Typhoid toxin belongs to the bacterial AB toxin family and consists of two enzymatic ‘A’ subunits, CdtB (cytolethal distending toxin A subunit; nuclease) and PltA (pertussis-like toxin A subunit; mono ADP-ribosyltransferase) linked to a homopentamer of receptor-binding ‘B’ subunit PltB (pertussis-like toxin B subunit), resulting in its unique A2B5 configuration. PltB recognizes the specific trisaccharide motif as its receptor, N-acetylneuraminic acid (Neu5Ac) α2–3 or α2–6 linked to the underlying disaccharide, galactose (Gal) β1-3/β1–4 linked N-acetylglucosamine (GlcNAc) or glucose. The pentameric configuration of the receptor-binding PltB subunit per toxin and the three glycan binding pockets per PltB monomer play an essential role for multivalent interactions between the toxin PltB and glycan receptor moieties. We previously revealed the three glycan-binding sites (BS) per PltB monomer and demonstrated the flexible use of these three binding sites in accommodating glycan receptor moieties that are structurally different.

We also solve co-crystal structures of PltB homopentamer bound to Neu5,9Ac2α2-6Galβ1-4GlcNAc and compare the glycan-binding interface with that for unmodified glycan counterparts. Both unmodified and 9-O-acetylated α2–6 glycans bind only to the BS1. 9-O-acetylated α2–6 glycans bound only to the BS1, while 9-O-Ac α2–3 glycans bound to the BS1 and BS2. Notable differences between the two are H-bonds between the 9-O-acetyl group and Thr65 (via the main chain), as well as between GlcNAc and Lys59 in the interface for 9-O-acetylated α2–6 glycans. These results are in support of the increased binding affinity of PltB to 9-O-acetylated α2–6 sialosides, compared to unmodified α2–6 counterpart. PltB binds to 9-O-acetylated α2–3 glycans (Neu5,9Ac2α2-3Galβ1-4GlcNAc) with a ~14-fold increased affinity compared to its unmodified α2–3 counterpart (Neu5Acα2-3Galβ1-4GlcNAc), while PltB binds to 9-O-acetylated α2–6 glycans (Neu5,9Ac2α2-6Galβ1-4GlcNAc) with a slightly higher affinity than its binding to unmodified α2–6 counterpart (Neu5Acα2-6Galβ1-4GlcNAc). Similar to PltB pentamer bound to unmodified glycan receptor moieties, we did not observe conformational changes of PltB pentamer bound to O-acetylated counterparts, compared to PltB protomer of typhoid holotoxin.

>EWTGDNTNAYYSDEVISELHVGQIDTSPYFCIKTVKANGSGTPVVACAVSKQSIWAPSFKELLDQARYFYSTGQSVRIHVQKNIWTYPLFVNTFSANALVGLSSCSATQCFGPK[5x]> GLEAAVDAAYEILLEELEKHGVRTIVVVGTGELALVLALAGVRLARERGVKTIVLVRDAAAAHRLLAALAAALGLPAPASADAAALAAADAALWAEHGLRVRVADLTDPAALRAALEALFAEHGRDDTLVLPAGEAALAALEPVLRELGLE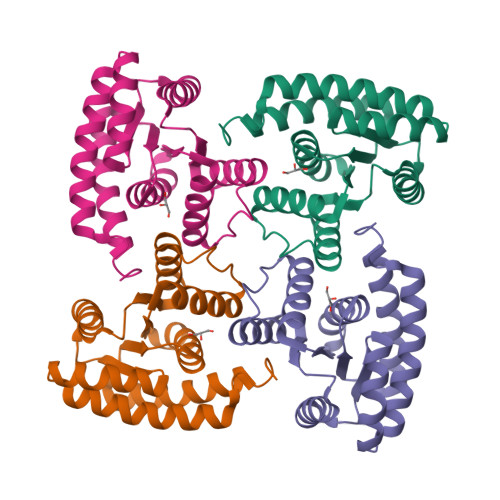EMAAVAREVYARLRAALAAARALEHHHHHHYARLRAALAAARALEHHH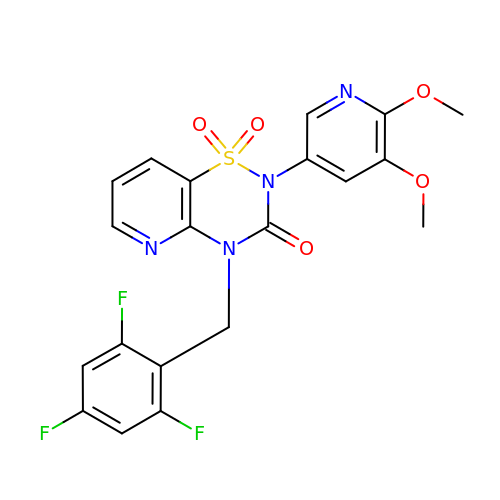2-(5,6-dimethoxypyridin-3-yl)-1,1-bis(oxidanylidene)-4-[[2,4,6-tris(fluoranyl)phenyl]methyl]pyrido[2,3-e][1,2,4]thiadiazin-3-one | C20 H15 F3 N4 O5 S | SUQZCEUKWPKXEE-UHFFFAOYSA-N The enzyme LkcE from the lankacidin polyketide biosynthetic pathway of the bacterium Streptomyces rochei represents an interesting test case for understanding such gain-of-function, as it exhibits a monoamine oxidase (MAO) protein fold yet also carries out a macrocyclization reaction. The catalytic mechanism proposed for LkcE involves initial oxidation of the amide function of LC-KA05 to an iminium ion. This is followed by attack of a C-2 enolate anion on the iminium to give the 17-membered lankacidinol A (2)8—an enzymatic intramolecular Mannich reaction.

In order to obtain complexes with LC-KA05, mutants E64A, E64Q, Y182F, R326L, and R326Q were soaked with the 1/7 substrate mixture followed by rapid acquisition of the X-ray diffraction data (owing both to the low availability of LC-KA05 and its high instability, it was not possible to carry out co-crystallization experiments). Of the five mutants, only E64Q and R326Q yielded co-complexes with 1; 7 was not observed in the active sites, as the acetate of 1 was clearly visible. The structure of the LkcE E64Q/LC-KA05 complex was solved at 3.03 Å resolution and that of the LkcE R326Q/LC-KA05 complex at 2.50 Å resolution by molecular replacement, using the structure of the LkcE/EMAA/DATD complex as the search model, and the presence of LC-KA05 confirmed using a weighted Fo−Fc omit map. In the E64Q structure in which R326 is present, the protein is identical, but the substrate adopts an alternative orientation, which allows it to interact with R326 (3.1 Å between the C-23 carbonyl of LC-KA05 and the R326 side chain). In both structures obtained in the presence of 1, the observed linear configuration of the polyketide chain would not permit subsequent cyclization involving the C-2 and C-18 centers (they are separated by 13.2 Å). This observation is consistent with the idea that LC-KA05 bound into the E64Q and R326Q mutants represents an on-pathway, pre-cyclization conformation. The side chain of E64 would then initiate ring closure by acting as a general base catalyst to activate the enol (there is no counterpart of this residue, to our knowledge, in other MAO family members). This key role is supported by the complete loss of activity seen with the E64A and E64Q mutants.

>[2x]GPGSMTVVEAKSRIAVVGGGGSGSVAAWLLARRHDVTLFEADEYLGGHAYSHPVETDQGTLHVDMGVQHFNEKLSPNLFRLLTDFGIGTYVAPSSVHVDFPGEQQSWNNLDFLGELREELHEEFDRFHQEMNQLPTSGDDSYKQMSIGEYLDKHGYSKSFKYKAMNPILSIYSGCHAPSLDYNLMYVALSFSMNLLSFFSAGYWRKAQGGIHSYLARIESDLGERVRLNTPVEAVVPTQSGVTVLAGGQEHHFDQVVFATHADVTLRLLRTSDQQYRDLLGDFAYVPVESVLHQDESWLSPAGGGAYCQFRMPEGFELARAEEQMGSLTRNCNVLHPYRKVSSPILITFDPQEDVDPERVIVRREWKLPQLRPVDVRRKKRLHEIQGLNGLWFCGTDTSVTGHEGAIVSGMVIADRLGVPHPFPDDAPAAAQFRGIKEFMGV>[3x]GSKKWFSEF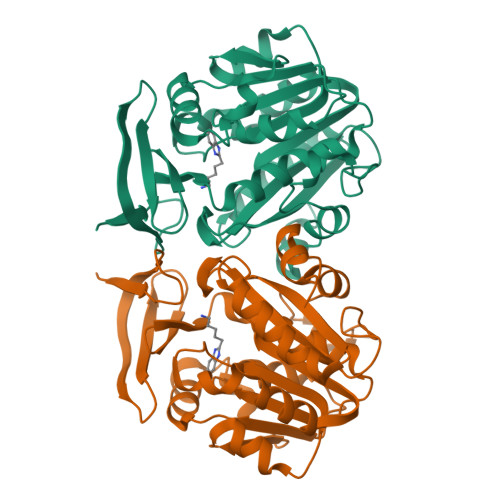SIMWPGQAFSLKIKKILYETKSKYQNVLVFESTTYGKVLVLDGVIQLTEKDEFAYHEMMTHVPMTVSKEPKNVLVVGGGDGGIIRELCKYKSVENIDICEIDETVIEVSKIYFKNISCGYEDKRVNVFIEDASKFLENVTNTYDVIIVDSSDPIGPAETLFNQNFYEKIYNALKPNGYCVAQCESLWIHVGTIKNMIGYAKKLFKKVEYANISIPTYPCGCIGILCCSKTDTGLTKPNKKLESKEFADLKYYNYENHSAAFKLPAFLLKEIENI1-[4-(3-chlorophenyl)phenyl]carbonyl-4-[2-(4-phenylmethoxyphenyl)ethanoylamino]piperidine-4-carboxylic 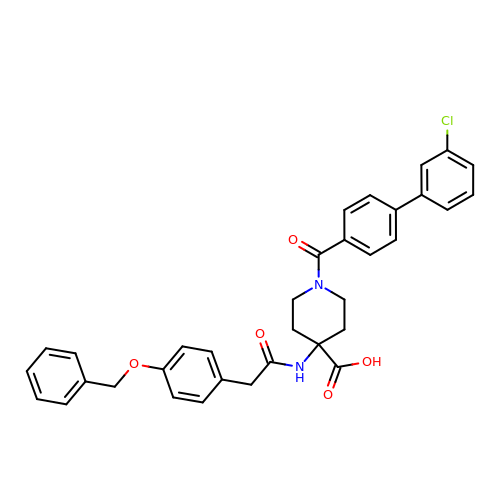acid | C34 H31 Cl N2 O5 | GRMOWKNKIVEDRP-UHFFFAOYSA-N As the multifunctional protein within the Flaviviridae family, Non-structural protein 1 (NS1) is considered as a promising target against flaviviruses. Moreover, the sNS1 lipoprotein is involved in virion production, immune evasion, and multiple aspects of pathogenesis. The NS1 monomer has 352 amino acids, forms 2 α-helices and 20 β-strands, and contains 12 conserved cysteine residues that form 6 intramolecular disulfide bonds. The NS1 monomer consists of three distinct domains: a β-roll domain (residues 1–29, β1–2), a wing domain (residues 38–151, β4–7 and α1–2), and a β-ladder domain (residues 181–352, β10–20). β3, β8, and β9 are from a ‘‘connector’’ domain (residues 30–37 and 152–180) and connect the wing to the β-roll and β-ladder domains.

The cryoEM structure of the YFV sNS1 tetramer is determined at a global resolution of 3.57 Å and is further improved to 3.31 Å by focusing the refinement on one of the dimers. The local resolution map shows that one of the dimers is blurry with a worse resolution, indicating its flexibility. Then, we performed focused refinement by applying a mask on one of the dimers and improved the resolution to 3.31 Å. The atomic models of the YFV_NS1_tetramer and focused refined dimer were built according to the density map. The chains were named AaBb and Aa for NS1 tetramer and dimer, respectively. Generally, all flavivirus NS1 dimers have a cross shape, formed by the intertwining of Monomer A and a, showing two distinct surfaces. The β-roll domain, the greasy finger (loopβ8–β9), and loopβ5–β6 in the wing periphery region form the ‘inner’ hydrophobic face, while the wing domain and β-ladder form the outer surface. In addition, we also use the Alpha fold to generate the 3D model of the YFV NS1 dimer. The structural comparison showed that the RMSD of the two dimers structures is 0.847 Å, suggesting the modelled dimer structure is very similar to that of the YFV_NS1 dimer.

>[2x]DQGCAINFGKRELKCGDGIFIFRDSDDWLNKYSYYPEDPVKLASIVKASFEEGKCGLNSVDSLEHEMWRSRADEINAIFEENEVDISVVVQDPKNVYQRGTHPFSRIRDGLQYGWKTWGKNLVFSPGRKNGSFIIDGKSRKECPFSNRVWNSFQIEEFGTGVFTTRVYMDAVFEYTIDCDGSILGAAVNGKKSAHGSPTFWMGSHEVNGTWMIHTLEALDYKECEWPLTHTIGTSVEESEMFMPRSIGGPVSSHNHIPGYKVQTNGPWMQVPLEVKREACPGTSVIIDGNCDGRGKSTRSTTDSGKVIPEWCCRSCTMPPVSFHGSDGCWYPMEIRPRKTHESHLVRSWVTAHHHHHH> SVIEFGKMIQEETDKNPLTSYSF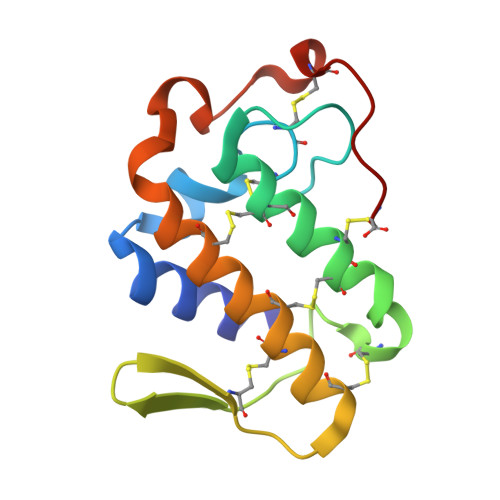YGCHCGLGNKGKPKDATDRCCFVHSCCYAKLSDCSPKTNRYEYHRENGAIVCGSSTPCKKQICECDRAAAICFRENLKTYNKKYKVYLRFKCKGVSEKC N-[(R)-1-benzothiophen-2-yl(2-chlorophenyl)methyl]-3,4-dihydro-2H-1,5-benzodioxepine-7-sulfonamide | C24 H20 Cl N O4 S2 | 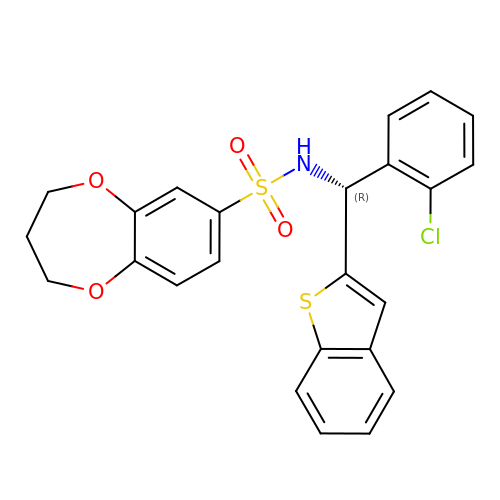TYGYAUYMFQMBTE-XMMPIXPASA-N> SCDTVDQGYQCFSETSHLWGQYAPFFSLANESVISPEVPAGCRVTFAQVLSRHGARYPTDSKGKKYSALIEEIQQNATTFDGKYAFLKTYNYSLGADDLTPFGEQELVNSGIKFYQRYESLTRNIVPFIRSSGSSRVIASGKKFIEGFQSTKLKDPRAQPGQSSPKIDVVISEASSSNNTLDPGTCTVFEDSELADTVEANFTATFVPSIRQRLENDLSGVTLTDTEVTYLMDMCSFDTISTSTVDTKLSPFCDLFTHDEWI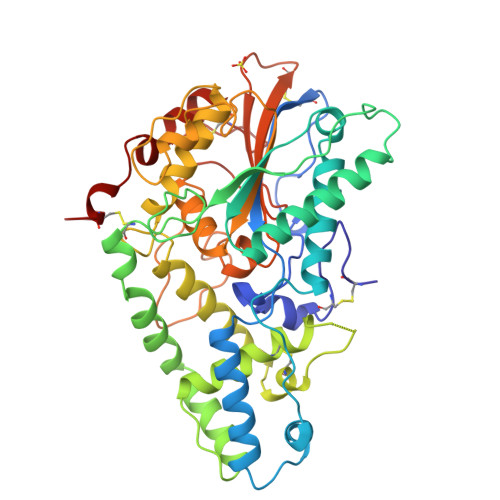NYDYLQSLKKYYGHGAGNPLGPTQGVGYANELIARLTHSPVHDDTSSNHTLDSSPATFPLNSTLYADFSHDNGIISILFALGLYNGTKPLSTTTVENITQTDGFSSAWTVPFASRLYVEMMQCQAEQEPLVRVLVNDRVVPLHGCPVDALGRCTRDSFVRGLSFARSGGDWAECFA> EDKCSPSGAICSGFGPPE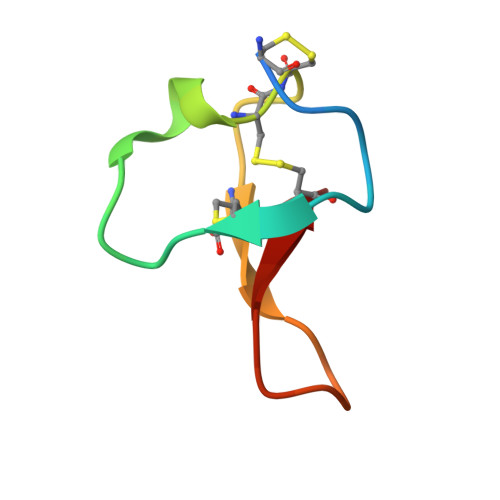QCCSGACVPHPILRIFVCQ>GEIPTIGQQMETGDQRFGDLVFRQLAPNVWQHTSYLDMPGFGAVASNGLIVRDGGRVLVVDTAWTDDQTAQILNWIKQEINLPVALAVVTHAHQDKMGGMDALHAAGIATYANALSNQLAPQEGMVAAQHSLTFAANGWVEPATAPNFGPLKVFYPGPGHTSDNITVGIDGTDIAFGGCLIKDSKAKSLGNLGDADTEHYAASARAFGAAFPKASMIVMSHSAPDSRAAITHTARMADKLR[2x]

BLs are categorised in two distinct families, according to their catalytic mechanism, and further divided into structural classes (Ambler’s classification): class A, C, and D serine β-lactamases (SBLs), which utilize a catalytic serine for β-lactam hydrolysis, and class B metallo-β-lactamases (MBLs), which, in turn, require divalent zinc ions for catalysis. Finally, subclass B1 MBLs inactivate nearly all β-lactam antibiotics, with the sole exception of monobactams. This class includes variants such as IMP-1, VIM-2 and NDM-1, whose worldwide emergence has characterized recent decades. Here, we present the identification of a series of non-covalent scaffolds targeting SBLs and concomitantly MBLs, through a large virtual screening study, in vitro validation, microbiological analysis and X-ray crystallography.

High-resolution structures of compounds 24 and 31 in complex with VIM-2 and NDM-1 MBL have been determined by single-crystal X-ray diffraction at 1.60 and 1.38 Å resolution, respectively. In the binary structures with NDM-1 compound 31 orients similarly to 24, with which it shares the same sulfhydryl-triazole moiety. With respect to 24 in VIM-2, compound 31 in NDM-1 is further stabilized by hydrophobic interactions formed with Ile28/35, Val67/73 and His263/250, and by a hydrogen bond with Gln119/123. The zinc ions maintain the position they have in the apo form, as well as the coordinating residues, i.e. His116/120, His118/122, Asp120/124, His196/189, Cys221/208, His263/250. In particular, in the case of NDM-1 they experience a slight opening upon binding of the inhibitors, while in VIM-2 their position appears quite conserved. For compound 31, the pose selected during the virtual screening was actually the one most similar to the crystallographic pose but was not the one that received the highest score in silico. It should be noted that the amide sidechain of Gln119/123 is flipped in the X-ray binary complex compared to the structure used for docking simulations, allowing it to interact with the ligand pyridyl nitrogen. We can observe a slight shift towards His196/189, possibly because of the flipped Gln119/123 or, alternatively, for the absence of water molecules in docking simulations. The highest ranking was, instead, assigned to a conformation of compound 31 having the opposite orientation with respect to the crystallographic one. The most potent compound is 31, which demonstrates an inhibition percentage of 97%.>SMDPERRVRSTLKKVFGFDSFKTPLQESATMAVVKGNKDVFVCMPTGAGKSLCYQLPALLAKGITIVVSPLIALIQDQVDHLLTLKVRVSSLNSKLSAQERKELLADLEREKPQTKILYITPEMAASSSFQPTLNSLVSRHLLSYLVVDEAHCVSQWGHDFRPDYLRLGALRSRLGHAPCVALTATATPQVQEDVFAALHLKKPVAIFKTPCFRANLFYDVQFKELISDPYGNLKDFCLKALGQEADKGLSGCGIVYCRTREACEQLAIELSCRGVNAKAYHAGLKASERTLVQNDWMEEKVPVIVATISFGMGVDKANVRFVAHWNIAKSMAGYYQESGRAGRDGKPSWCRLYYSRNDRDQVSFLIRKEVAKLQEKRGNKASDKATIMAFDALVTFCEELGCRHAAIAKYFGDALPACAKGCDHCQNPTAVRRRLEALERSSSW[4x]

RECQL5 (also known as RECQ5) is a member of the RecQ family of helicases, which are highly conserved throughout evolution, and function in many diverse cellular processes with the role of maintaining genome integrity. Specific roles have been established for RECQL5 in almost every cellular process involving DNA, including transcription, replication, recombination, chromosomal segregation and DNA repair. The Zn2+-binding domain consists of a pair of long antiparallel α-helices (also known as the helical hairpin), followed by series of short helices and loops, from which a cluster of cysteine residues bind in a typical Cys4 tetrahedral arrangement to a single Zn2+ ion.

In an attempt to improve the diffraction properties of these crystals a new construct spanning residues 11–453 was produced and crystallization experiments were set up with and without nucleotides as above. In this case crystals were obtained in complex with the nucleotide ADP/Mg2+ in two different crystal forms, both of which diffract to significantly higher resolution (1.8 Å for the monoclinic crystals, and 2.0 Å for the triclinic). The ADP bound structures were solved by molecular replacement using the APO form as a search model, with two RECQL5 monomers in the asymmetric unit of the monoclinic crystals, and four copies in the triclinic crystals. In both cases, the electron density maps are of excellent quality throughout and the structures are very similar, although slight differences remain in the domain orientation and conformation of various loops which are discussed in more detail below. Similar but less dramatic differences can be seen when comparing the six independent chains of the two ADP crystal forms, which can be grouped into two distinct clusters of three which are separated by maximum displacements of up to 9 Å. Looking at residues at the interface between the two domains, a clear correlated difference can be seen in the conformation of residues forming the aromatic rich loop (AR loop). In the more open form H167 and D168 are pointing toward motif II, making water-mediated interactions with T194 and H160 (conserved residues from motifs III and II respectively), while in the less open form H167 is pointing away from motif II, forming a water-mediated interaction with Y419 (part of the Zn2+ binding domain). In the ADP complex, the ADP moiety is bound in the active site, making extensive interactions with residues in the D1 domain, several of which belong to the conserved helicase motifs Q, I and II. The most prominent difference is in the relative orientations of the D1 and D2 domains, with the inter-domain cleft almost completely closed in the APO form and considerably more open in the ADP bound form, with maximal displacements of equivalent residues of up to 30 Å.>[4x]MGSNVNAPRVRRSVRDLQKRYDNGEKKPLEDLVRAWVGIQALPPSDPKSFFALGGYHGEPFQYRKPVDALPQDDIYPYWGGYCNHGNVLFPTWHRMYVYKLEEALQSIVPGVSMPFWDETDEYTLKHGIPSILTQEKFELDGKQIDNPLRSFVLPVALSDRLPGDGNIYEKPKGYVTVRYPLSGLVGTPEALEQTKIHNAKFPLPEKNTELLNSNVRAWLKGDSPTPGDPDPTRNGVYAKYVRCLSAPNYTVFSNTTSASVWNS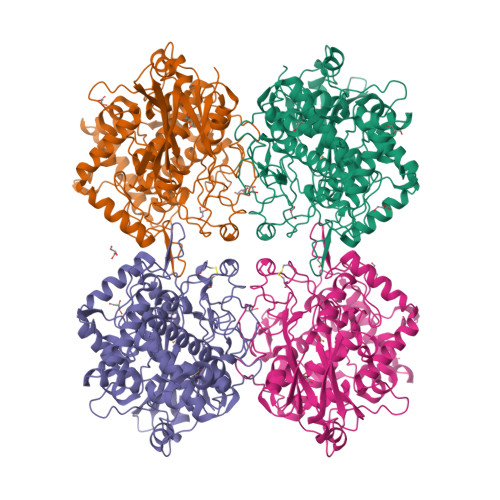SNPGLVTPVESPHNDIHLAVGGFDYGGDEIGQIAGANGDMGENNTAGMDPIFFFHHCNVDRMFWVWQKQTGHTDRLDIIRNYPGTNASDSQGPTPGFAPGESLNLTTPLNPFKKASGEAYTSEDCINIERQLGFTYGPGSLDDATPELKSLLAVPSGNSTKKLTVTGIDRAQIQGSFIMKAYASVTDANGKTREYYLGHKSILSRWNVVQCANCLTHLDIVAHFPLSAMPADDVPKAKFRVEFIHRGGGVPSAAKAAIDKVSALQPKFEVSDKLAAALEHHHHHH> GIEDLIDTAIKNALRVSQPPSTQSTEATSGVNSQEVPALTAVETGASGQAIPSDVVETRHVVNYKTRSESCLESFFGRAACVTILSLTNSSKSGEEKKHFNIWNI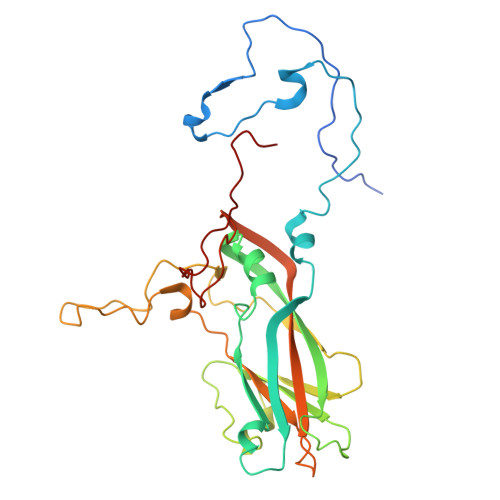TYTDTVQLRRKLEFFTYSRFDLEMTFVFTENYPSTASGEVRNQVYQIMYIPPGAPRPSSWDDYTWQSSSNPSIFYMYGNAPPRMSIPYVGIANAYSHFYDGFARVPLEGENTDAGDTFYGLVSINDFGVLAVRAVNRSNPHTIHTSVRVYMKPKHIRCWCPRPPRAVLYRGEGVDMISSAILPLTKVDSITTF>YECRIQRLTAQEPQYRLEAEAGVSEVWDYTDQQFRCAGVAALRNTIRPQGLLLPVYTNAPKLYYVTQGRGILGVLMPGCPETFQSMSQFQGSREQEEERGRFQDQHQKVHHLKKGDIIAIPAGVALWCYNDGDEDLVTVLVQHTASDLNQLDQNPRHFFLAGNIQRSQKQRGERYGLRGGQQILADNVFKGFNMEALADVLGFGMDTETARKVRGEDDQRGHIVRVEQGLKVIRPPRIREELEQQEGGGYNGLEETICSATFIQNIDNPAEADFYNPRAGRLTTVNSLKVPILTFLQLSAMKGVLYENAMMAPLWRLNANSVVYAVRGEARVQIVDHRGETV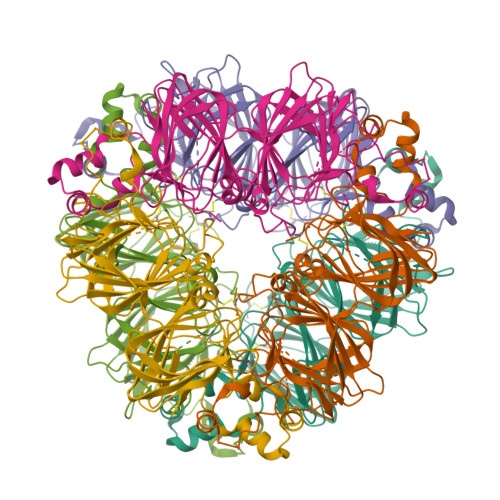FDDNLREGQMVVVPQNFVVVKQAGSRGFEWVVFNTNDNALFSTAAGRTSPLRGIPVGVLANAYRLSQEEARRIKLNRDEAVLFN[2x]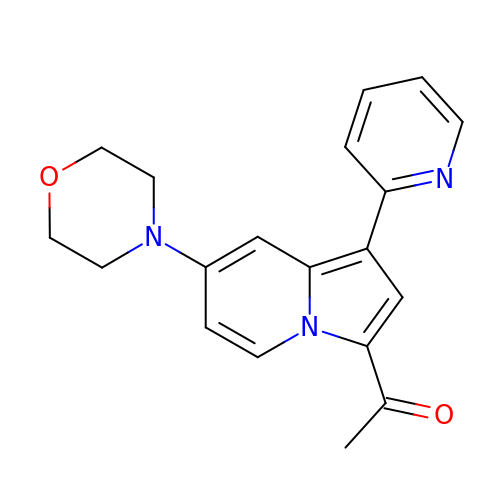1-[7-(morpholin-4-yl)-1-(pyridin-2-yl)indolizin-3-yl]ethanone | C19 H19 N3 O2 | JNCJVBDKESBLNW-UHFFFAOYSA-N4-{[(1R,2S)-1,2-dihydroxy-2-methyl-3-(4-nitrophenoxy)propyl]amino}-2-(trifluoromethyl)benzonitrile | C18 H16 F3 N3 O5 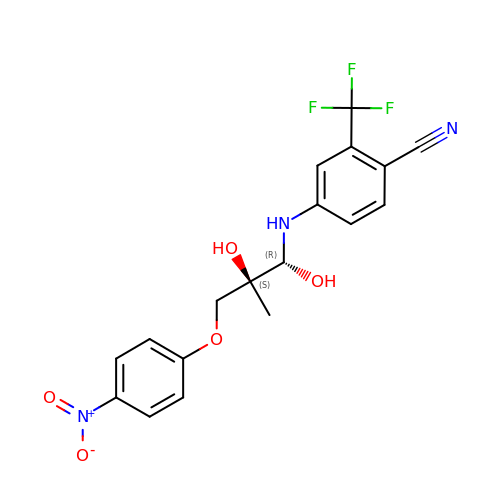| INVUBEGZQHQAMY-SJORKVTESA-N> ASGVADDMACHKIPVEADFLYAYSTAPGYYSWRNSKDGSWFIQSLCAMLKQYADKLEFMHILTRVNRKVATEFESFSFDATFHAKKQIPCIVSMLTKELY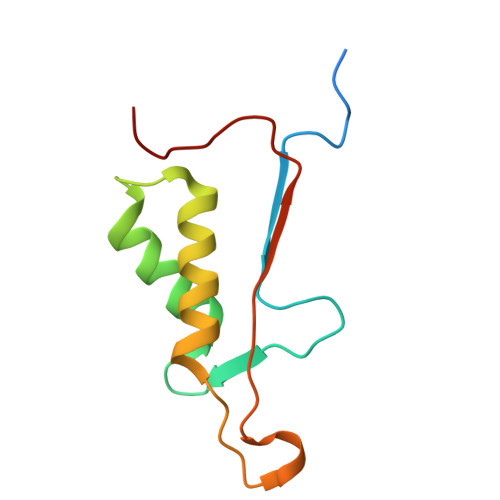FYH> AARYDDILYFPASRYPETGAHISDAIKAGHSDVCTIERSGADKRRQESLKGIPTKPGFDRDEWPMAMCEEGGKGASVRYVSSSDNRGAGSWVGNRLSGFA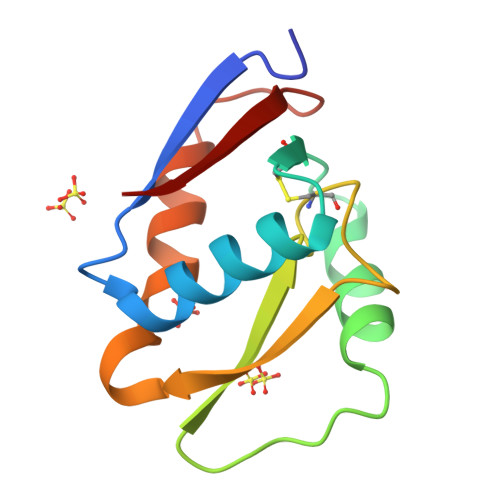DGTRILFIVQ>MKTIKDRIAKWSAIGLLSAVAATAFYAPSASAHGEKSQAAFMRMRTIHWYDLSWSKEKVKINETVEIKGKFHVFEGWPETVDEPDVAFLNVGMPGPVFIRKESYIGGQLVPRSVRLEIGKTYDFRVVLKARRPGDWHVHTMMNVQGGGPIIGPGKWITVEGSMSEFRNPVTTLTGQTVDLENYNEGNTYFWHAFWFAIGVAWIGYWSRRPIFIPRLLMVDAGRADELVSATDRKVAMGFLAATILIVVMAMSSANSKYPITIPLQAGTMRGMKPLELPAPTVSVKVEDATYRVPGRAMRMKLTITNHGNSPIRLGEFYTASVRFLDSDVYKDTTGYPEDLLAEDGLSVSDNSPLAPGETRTVDVTASDAAWEVYRLSDIIYDPDSRFAGLLFFFDATGNRQVVQIDAPLIPSFM[3x];>MSAAQSAVRSHAEAVQVSRTIDWMALFVVFFVIVGSYHIHAMLTMGDWDFWSDWKDRRLWVTVTPIVLVTFPAAVQSYLWERYRLPWGATVCVLGLLLGEW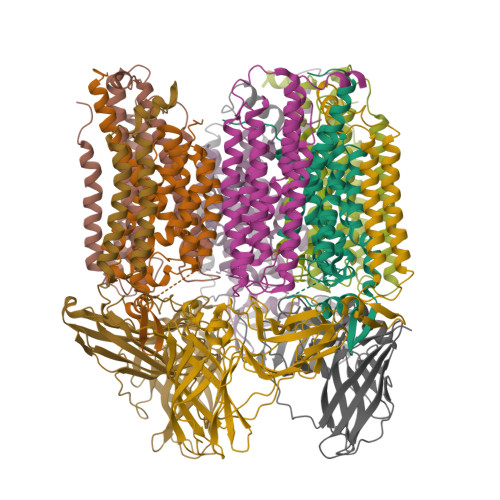INRYFNFWGWTYFPINFVFPASLVPGAIILDTVLMLSGSYLFTAIVGAMGWGLIFYPGNWPIIAPLHVPVEYNGMLMSIADIQGYNYVRTGTPEYIRMVEKGTLRTFGKDVAPVSAFFSAFMSILIYFMWHFIGRWFSNERFLQST[3x];>[3x]MHETKQGGEKRFTGAICRCSHRYNSMEVKMAATTIGGAAAAEAPLLDKKWLTFALAIYTVFYLWVRWYEGVYGWSAGLDSFAPEFETYWMNFLYTEIVLEIVTASILWGYLWKTRDRNLAALTPREELRRNFTHLVWLVAYAWAIYWGASYFTEQDGTWHQTIVRDTDFTPSHIIEFYLSYPIYIITGFAAFIYAKTRLPFFAKGISLPYLVLVVGPFMILPNVGLNEWGHTFWFMEELFVAPLHYGFVIFGWLALAVMGTLTQTFYSFAQGGLGQSLCEAVDEGLIAK>PPNEITLTIGQQKDLASMVPAKFAGQELSWTSSDPETASVTDKGIVTALKFSSGGANLFLKAPATGEAIITVTAGKQSHSVKVITTVKGKEDIEKLPPLKDHFKDYFLIGNIFNNRDVSGSMMDNDWLAHHYAILTPENHMKPSNLTNNRNETTGEITYTFSTADRMVNAAIAEGLKIHGHTLLWHQQIPPWQRSMESAAKDAALSVMKKYITEVMTHYKGKIYSWDVLNEIFPDGRGDNWTTAMRPENPWFKSIGSDFVYEAYLAARQADPNAILYYNDYNMDQAGKAALIAAMVRDVN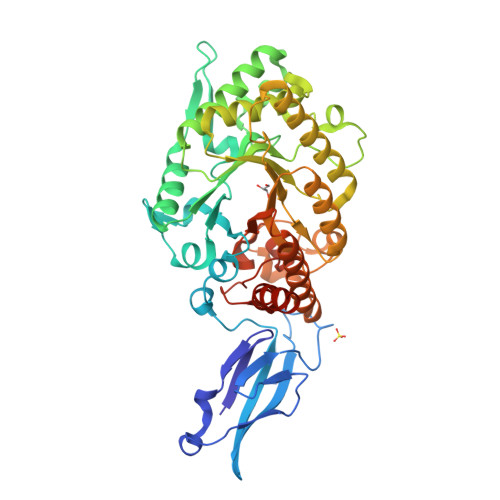AKYKQAYPRETRLLIEGIGMQSHHNMDVPASNIRNTINRYRELGVKISVSELDILCMGWSAFRGSTGQGADKDDMTIATNRNILDQAYKFNEYMKLYLENSDIIERVSMWGVSDRYSWRSGGLPLLFDADNKAKPAYYSFVRAREDYEAAKAAKAE[8x]> ARVTVQDAVEKIGNRFDLVLVAARRARQMQVGGKDPLVPEENDKTTVIALREIEEGLINNQILD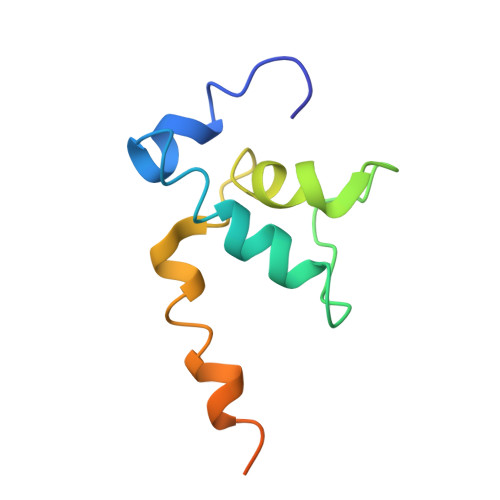VRERQEQQEQEAAELQAVTAIAEGRR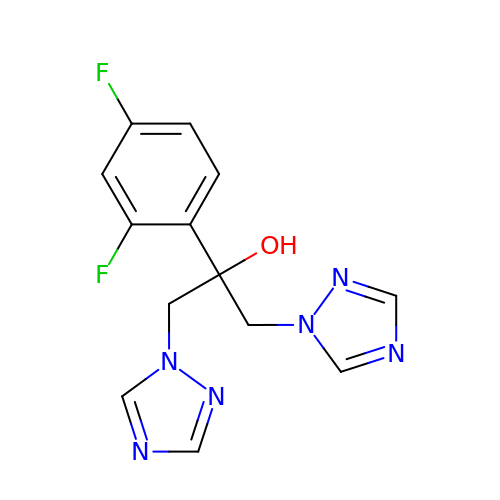2-(2,4-DIFLUOROPHENYL)-1,3-DI(1H-1,2,4-TRIAZOL-1-YL)PROPAN-2-OL | C13 H12 F2 N6 O | RFHAOTPXVQNOHP-UHFFFAOYSA-N>MASVQLQNVTKAWGEVVVSKDINLDIHEGEFVVFVGPSGCGKSTLLRMIAGLETITSGDLFIGEKRMNDTPPAERGVGMVFQSYALYPHLSVAENMSFGLKLAGAKKEVINQRVNQVAEVLQLAHLLDRKPKALSGGQRQRVAIGRTLVAEPSVFLLDEPLSNLDAALRVQMRIEISRLHKRLGRTMIYVTHDQVEAMTLADKIVVLDAGRVAQVGKPLELYHYPADRFVAGFIGSPKMNFLPVKVTATAIDQVQVELPMPNRQQVWLPVES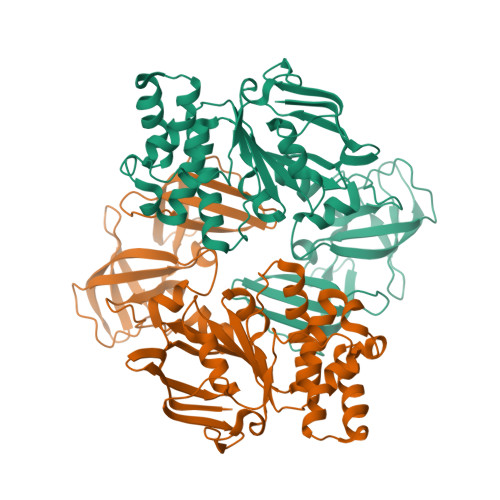RDVQVGANMSLGIRPEHLLPSDIADVILEGEVQVVEQLGNETQIHIQIPSIRQNLVYRQNDVVLVEEGATFAIGLPPERCHLFREDGTACRRLHKEPGVASASHHHHHH[2x]> MTDDKDVLRDVWFGRIPTCFTLYQDEITEREAEPYYLLLPRVSYLTLVTDKVKKHFQKVMRQEDISEIWFEYEGTPLKWHYPIGLLFDLLASSSALPWNITVHFKSFPEKDLLHCPSKDAIEAHFMSCMKEADALKHKSQVINEMQKKDHKQLW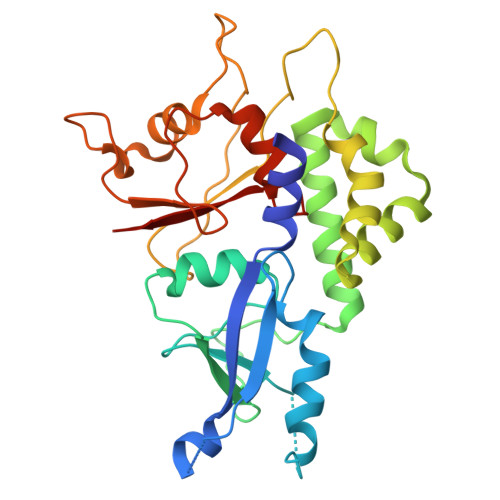MGLQNDRFDQFWAINRKLMEYPAEENGFRYIPFRIYQTTTERPFIQKLFRPVAADGQLHTLGDLLKEVCPSAIDPEDGEKKNQVMIHGIEPMLETPLQWLSEHLSYPDNFLHISIIPQPTD> MERFLRKYNISGDYANATRTFLAISPQWTCSHLKRNCLFNGMCAKQNFERAMIAATDAEEPAKAYRLVELAKEAMYDRETVWLQCFKSFSQPYEEDIEGKMKRCGAQLLEDYRKNGM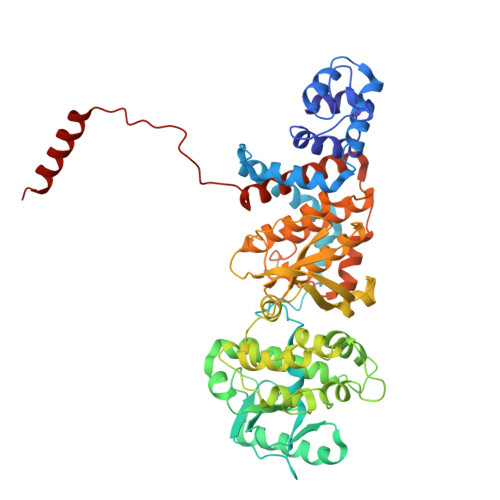MDEAVKQSALVNSERVRLDDSLSAMPYIYVPIKEGQIVNPTFISRYRQIAYYFYSPNLADDWIDPNLFGIRGQHNQIKREIERQVNTCPYTGYKGRVLQVMFLPIQLINFLRMDDFAKHFNRYASMAIQQYLRVGYAEEVRYVQQLFGKIPTGEFPLHHMMLMRRDFPTRDRSIVEARVRRSGDENWQSWLLPMIIVREGLDHQDRWEWLIDYMDRKHTCQLCYLKHSKQIPTCGVIDVRASELTGCSPFKTVKIEEHVGNNSVFETKLVRDEQIGRIGDHYYTTNCYTGAEALITTAIHIHRWIRGCGIWNDEGWREGIFMLGRVLLRWELTKAQRSALLRLFCFVCYGYAPRADGTIPDWNNLGSFLDTILKGPELSEDEDERAYATMFEMVRCIITLCYAEKVHFAGFAAPACESGEVINLAARMSQMRMEY An essential structural component of bacterial biofilms is functional amyloid (FuA), which also has great potential as an engineerable nano‐biomaterial. The two most well studied examples are the curli system in Escherichia coli and the fap system in Pseudomonas, in which the major aggregating protein is CsgA and FapC, respectively. A fully experimentally based 3.2 Å resolution cryo‐electron microscopy density map of the FuA protein FapC from Pseudomonas sp. UK4 is presented, which reveals a Greek key‐shaped protofilament. Each FapC monomer consists of three imperfect repeats (IRs), with each repeat forming one cross‐β layer.

We reprocessed the data using a 14.4 Å (3 × 4.8 Å) helical rise and −6° twist, corresponding to a monomer with 3 layers of cross‐β structure. When we performed 3D helical reconstruction, we obtained density maps at 3.2 Å which show great overall similarity between the three layers but with differences in details (Table 1 and Figures 4e and 6 and Figures S13 and S15a,b). A model of this FapC fibril was constructed by fitting the density map of three layers with the AF3 model which contains three IRs of FapC residues 45–96, 110–161, and 173–234, while loop linkers and other flexible region of the protein cannot be modeled due to poor electron density. Residues 45–96, 110–161, and 173–234 comprise the FapC fibril core of layers 1–3, respectively, excluding disordered residues 58–59 of IR1, 123–124 of IR2, and 186–197 of IR3 which form part of the core but do not show sufficiently high electron density to be mapped on the structure. The Greek key‐shaped cross‐β structure is composed of five short β‐strands, each layer spiraling around the helical axis. The Greek key‐shaped structure is formed with strands β4 and β5 tilting out‐of‐plane relative to β1, β2, and β3 along the fibril axis. The staggered structure of FapC fibril allows a residue from repeat layer (i) to interact with the neighboring residues in layers (i + 1) and (i − 1) within the same β‐sheet, and with residues at the opposite β‐sheet in layer (i) and (i − 1) or (i) and (i + 1) to form hydrogen bonding interactions. In addition to the many hydrophobic interaction in the core, the FapC fibril structure is stabilized by an extensive network of hydrogen bonds. More strikingly, the five highly conserved Asn/Gln polar residues located inside the inner core engage in extensive side chain hydrogen‐bonding in the inner core of the Greek key arch. The cryo‐EM structure suggests that Asn and Gln residues maintain the shape of the Greek key arch in the FapC fibril, which may explain their high conservation in the predicted structures of FapC family.

>MKPTMALKPLVFALAALMAVAAQAGPAEKWKPTPAPTGTVAAAVTDTQVSKDNKFDDTKTLNNAGANGSLSNSKGNLGANIAAGSGNQQDNAAAITSSAGDAATVFAVADIYQESKDNKFTNKGTQNNALLNNSANNSSGNVGVNVAAGQGNQQKNNLAIVTADGKNVAAASNTEQVSLDNHFLNEASSKHSYKPQYVVNNAGLLNSANNASGNIGVNVAAGAGNQQSNTLTLGSGCTVCAAGTGSKLAF[3x]>[6x]MALWQQGQKLYLPPTPVSKVLCSETYVQRKSIFYHAETERLLTIGHPYYPVSIGAKTVPKVSANQYRVFKIQLPDPNQFALPDRTVHNPSKERLVWAVIGVQVSRGQPLGGTVTGHPTFNALLDAENVNRKVTTQTTDDRKQTGLDAKQQQILLLGCTPAEGEYWTTARPCVTDRLENGACPPLELKNKHIEDGDMMEIGFGAAN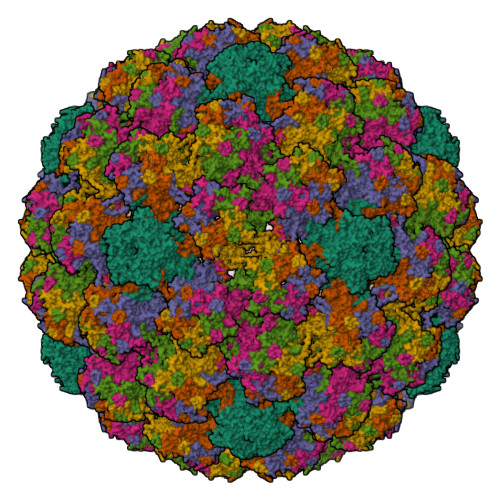FKEINASKSDLPLDIQNEICLYPDYLKMAEDAAGNSMFFFARKEQVYVRHIWTRGGSEKEAPTTDFYLKNNKGDATLKIPSVHFGSPSGSLVSTDNQIFNRPYWLFRAQGMNNGIAWNNLLFLTVGDNTRGTNLTISVASDGTPLTEYDSSKFNVYHRHMEEYKLAFILELCSVEITAQTVSHLQGLMPSVLENWEIGVQPPTSSILEDTYRYIESPATKCASNVIPAKEDPYAGFKFWNIDLKEKLSLDLDQFPLGRRFLAQQGAGCSTVRKRRISQKTSSKPAKKKKK URACIL | C4 H4 N2 O2 | 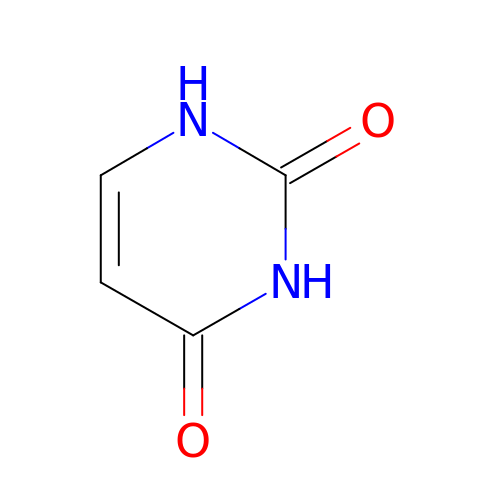ISAKRJDGNUQOIC-UHFFFAOYSA-N4-({[(2R)-2-methyl-2-(morpholin-4-yl)butyl]carbamoyl}amino)-N-(1,3-thiazol-2-yl)benzamide 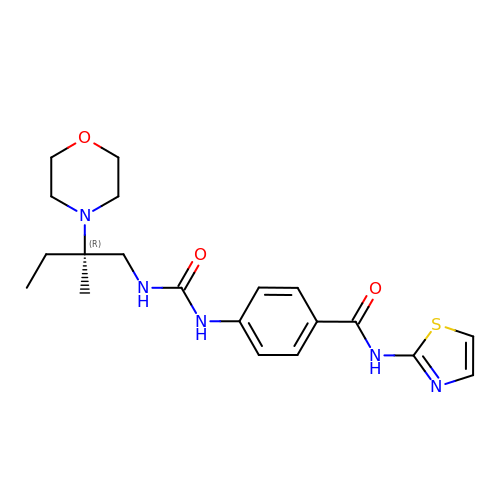| C20 H27 N5 O3 S | DBKPEQXYKJIJBQ-HXUWFJFHSA-N> SDHHHHHHGPISPIETVPVKLKPGMDGPKVKQWPLTEEKIKALVEICTEMEKEGKIS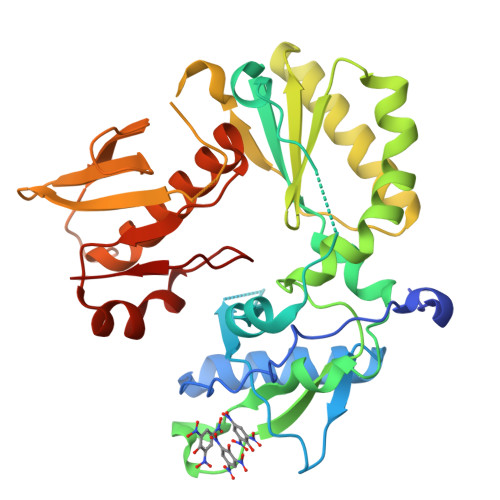KIGPENPYNTPVFAIKKKDSTKWRKLVDFRELNKRTQDFWEVQLGIPHPAGLKKKKSVTVLDVGDAYFSVPLDEDFRKYTAFTIPSINNETPGIRYQYNVLPQGWKGSPAIFQSSMTKILEPFKKQNPDIVIYQYMDDLYVGSDLEIGQHRTKISELRQHLLRWGLTTPDGYELHPDKWTGSGSGGYDPSKDLIAEIQKQGQGQWTYQIYQEPSKNLKTGKYARMRGAHTNDVKQLTEAVQKITTESIVIWGKTPKFKLPIQKETWETWWTEYWQATWIPEWEFVN>SKVLVLKSSILAGYSQSNQLSDYFVEQWREKHSADEITVRDLAANPIPVLDGELVGALRPSDAPLTPRQQEALALSDELIAELKAHDVIVIAAPMYNFNISTQLKNYFDLVARAGVTFRYTENGPEGLVTGKKAIVITSRGGIHKDGPTDLVTPYLSTFLGFIGITDVKFVFAEGIAYGPEMAAKAQSDAKAAIDSIVS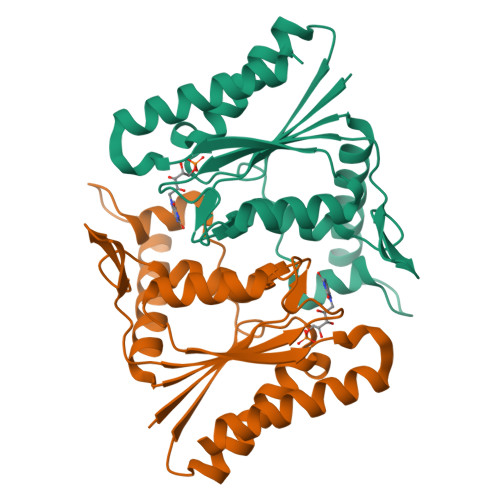A[2x]> YKDGDQCETSPCQNQGKCKDGLGEYTCTCLEGFEGKNCELFTRKLCSLDNGDCDQFCHEEQNSVVCSCARGYT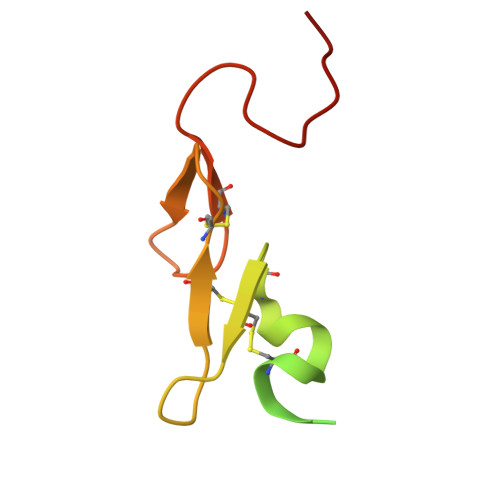LADNGKACIPTGPYPCGKQTLER>GSGLNIKENDLPGIGKKFEIETRSHEKMTIIIHDDGRREIYRFND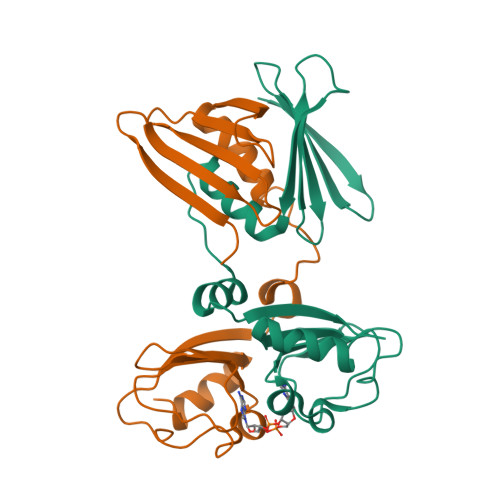RDPDELLSNISLDDSEARQIAAILGGMVYKPQALESIEMAFSDLIIEWFKVEKGAKSIGRTLGELDVRQNYDVTVIAIIKHNQEKLLNPGADSIIEENDTLVLSGERKHLKKLIHDFLSGEGV[4x]>MSKPQPIAAANWKCNGSQQSLSELIDLFNSTSINHDVQCVVASTFVHLAMTKERLSHPKFVIAAQNAIAKSGAFTGEVSLPILKDFGVNWIVLGHSERRAYYGETNEIVADKVAAAVASGFMVIACIGETLQERESGRTAVVVLTQIAAIAKKLKKADWAKVVIAYEPVWAIGTGKVATPQQAQEAHALISSWVSSKIGADVAGELRILYG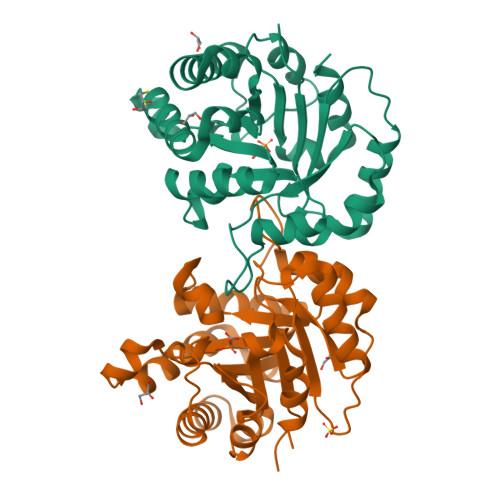GSVNGKNARTLYQQRDVNGFLVGGASLKPEFVDIIKATQ[2x]>[2x]ETAIPFSRRRMPYSLGTDKLEKVDPDKIKSKLSEDVERKLETDMRELYDRLLPTEAIEVNRRELVSKLERLFNTEWPGHDIRVHLFGSSGNLLCSDDSDVDICITTPWRELESVCMIAELLDRHGMEKVVCVSSAKVPIVKIWDPELKLACDMNVNNTLALENTRMVRTYVSIDDRVRPLAMIIKYWTRRRVVNDAAFGGTLSSYTWICMIIAFLQLRDPPVLPALHQQHDLKLVKQDGALSDFADDIPKLRGFGAKNKDSLAVLLFQFFRFYAHEFDYDKYTLSIRMGTLLTKAEKNWQYLVNNALCVEEPFNDGRNLGNTADETSFRGLHMELRRAFDLIAEGKLEECCEQYVFPKEEERV

Template-independent terminal ribonucleotide transferases (TENTs) catalyze the addition of nucleotide monophosphates to the 3′-end of RNA molecules regulating their fate. TENTs include poly(U) polymerases (PUPs) with a subgroup of 3′ CUCU-tagging enzymes, such as CutA in Aspergillus nidulans. CutA preferentially incorporates cytosines, processively polymerizes only adenosines and does not incorporate or extend guanosines. Here, we report structures of the catalytic core of T. terrestris CutA (TtCutA) in the apo form and its complexes with a non-hydrolyzable CTP analog and A3 RNA.

Therefore, based on in silico predictions, we designed over a dozen protein variants that were truncated up to predicted helices at both N- and C-termini and tested their expression and purification efficiency in a soluble and intact form. This approach eventually led to a TtCutA240–603 fragment that contained the catalytic core of the protein. We first obtained crystals of the apo form of the protein, the structure of which was solved by SeMet SAD and refined against a data set from native protein crystal to 2.25 Å resolution and an Rfree of 24.1%. The protein conformation in the apo state and in both complexes with nucleic acid is essentially the same. We observed small movements of the palm and finger domains relative to each other. As expected, the overall protein structure is very similar to other TENTs and adopts a bilobal architecture. The active site and incoming nucleotide are located between the palm and finger subdomains.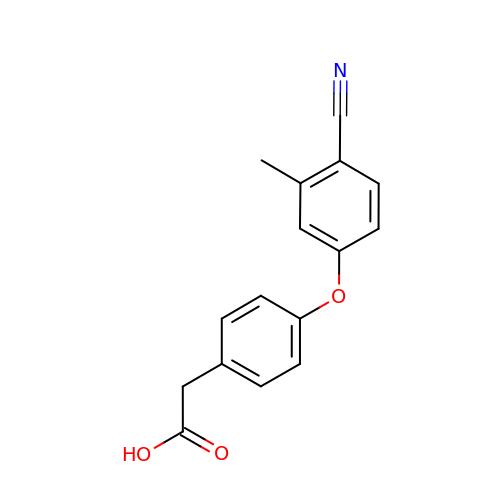[4-(4-cyano-3-methylphenoxy)phenyl]acetic acid | C16 H13 N O3 | VDBBDYPELPDNGF-UHFFFAOYSA-N2-(2-{2-[2-(2-METHOXY-ETHOXY)-ETHOXY]-ETHOXY}-ETHOXY)-ETHANOL | C11 H24 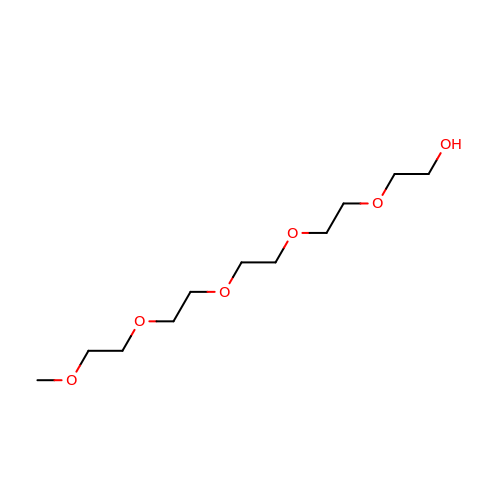O6 | SLNYBUIEAMRFSZ-UHFFFAOYSA-N>[2x]GSLSKVEESQLNEKENKNVADGLAWSYYFGYLKFVLPELEKQIEKTSKFRSKEKFVKKMFILIPSNCFWDDKIPGSDYDPQNRIT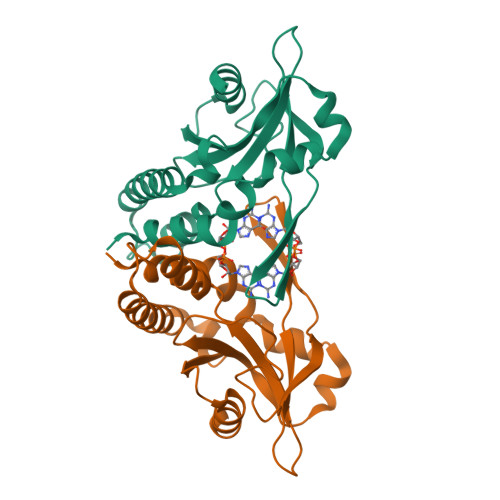FEGNTEPLEKTRGGVKLRHYKHSVYEIKDGENEPWFCIMEYATPLLTLYDMSVAQPGELSREERDAQVVVFLRKLQDILEGDRACQGKYELVTFSPDRDLADVMLRKLKDSELEIGG D-arabinohydroxamic acid | C5 H9 N O7 | 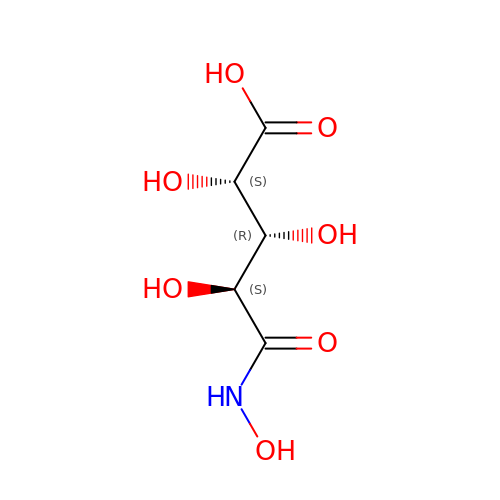DMGBHBFPSRKPBV-LAMMAJBHSA-N> HTPVRTVMNTIQQLMMILNSASDQPSENLISYFNNCTVNPKESILKRVKDIGYIFKEKFAKAVGQGCVEIGSQRYKLGVRLYYRVMESMLKSEEERLSIQNFSKLLNDNIFHMSLLACALEVVMATYSRSTSQNLDSGTDL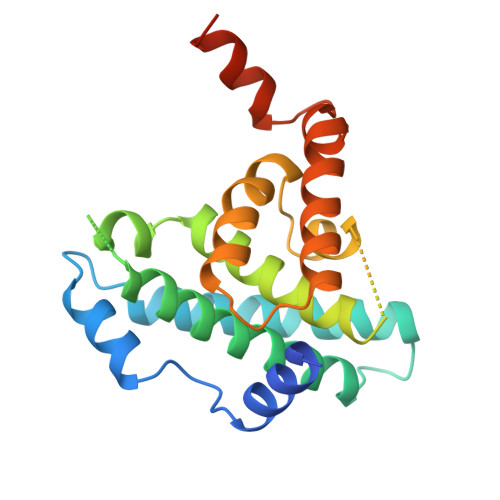SFPWILNVLNLKAFDFYKVIESFIKAEGNLTREMIKHLERCEHRIMESLAWLSDSPLFDLIKQSKDREGPTDHLESA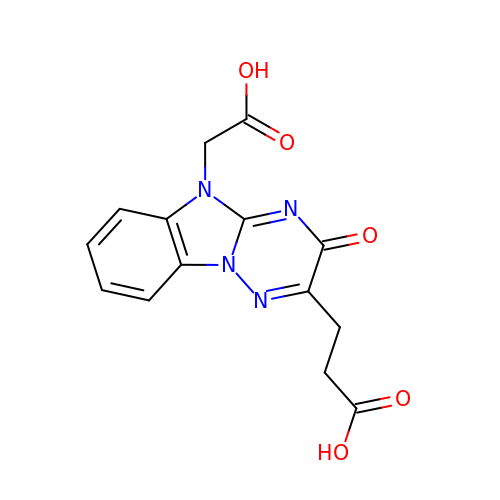3-[5-(2-hydroxy-2-oxoethyl)-3-oxidanylidene-[1,2,4]triazino[2,3-a]benzimidazol-2-yl]propanoic acid | C14 H12 N4 O5 | IBSCUNBMGSFHGD-UHFFFAOYSA-N>[3x]PAQTSVSELGFLCGMMRSRGLRKYIISHLSDVAKLREEVPAALKGAPKPAKLVLECIGRFFLQGSKAFGKATHMVPSRQASLLILEFFLLSDCTEMEPSVKEEADLAAVTWRKRLINEGGVSNASDIDARGLLLLVASFGIPALFRNEDL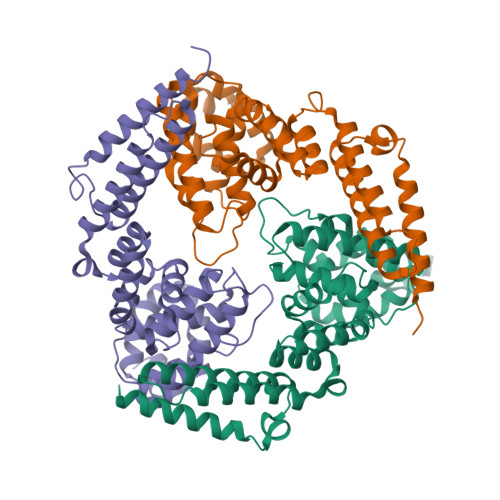RNLIRLSCPKEISDALRRSRFLLARVPDVIQGMIKNQMNVEAVDFAYTFGLEEKFPIWKILTSFLREHKEEWKRTREEDSPIRLKKANENYLSAMKSVTRCLEDHRVDPSKLLSGWHIDEKIIQLEKEMADLDKKMEGK Doxazosin, (S)- | C23 H25 N5 O5 | 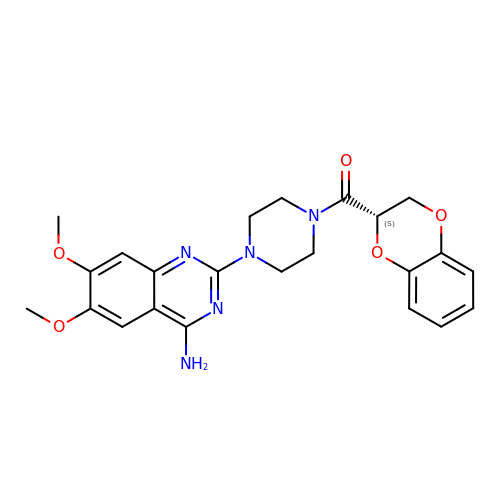RUZYUOTYCVRMRZ-FQEVSTJZSA-N~{N}-[(2~{S},3~{S},4~{S},5~{R})-2-(hydroxymethyl)-4,5,6-tris(oxidanyl)oxan-3-yl]-2-oxidanyl-ethanamide | C14 H27 N4 O9 | 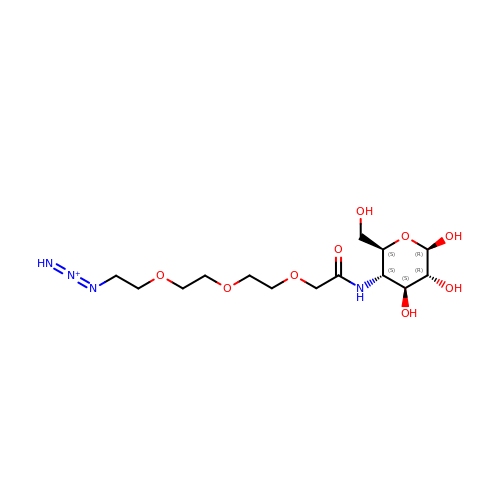RPRHCZBAXXPRCX-RGCYKPLRSA-O> YILPEDWHLRFPSGSEIIQYAASHYVKNSLDPDEQLLDRRRVEYDIFLLVEELHVLDIIRKGFGSVDEFIALANSVSNRRKSRAGKSLELHLEHLFIEHGLRHFATQAITEGNKKPDFLFPSAGAYHDTEFPVENLRMLAVKTTCKDRWRQILNEADKIHQVHLFTLQEGVSLAQYREMRESGVRLVVPSSLHKKYPEAVRA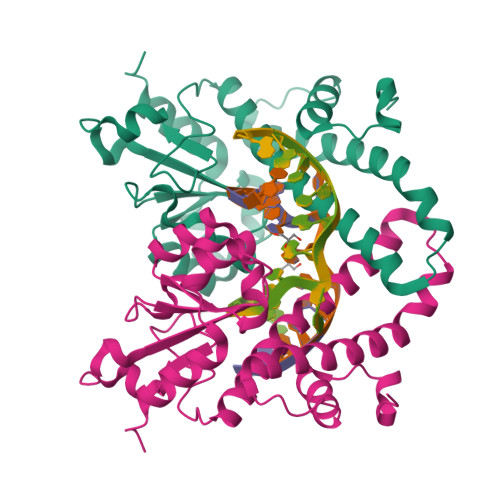ELMTLGAFIAELTGLYADIP>[2x]MELDKTKFREMYLQNDSRVDSYDGKMEYVWNGRISKDGDSGGVGLHTGTGTKDGPAVFTFDLGVLAKLSRFALWAIQDEKHFY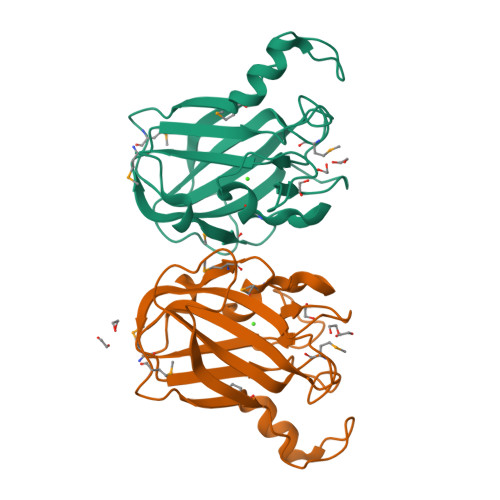NDMSPRRYEVWGCATEPNPDGSWDQWVKLLDMENVKPSGSPIGILTEDDIEAAKIGDQANVPLDMPRVRYIRIKCLKNWSNNYNICFTELTFWGND Four helix bundles are also attractive for synthetic chemists because its interfaces are dominated by side chain and side chain interactions, which can be more tunable than β-strands. This study focuses on TmFtn, a naturally dimeric protein consisting of two antiparallel four helix bundles, as shown in Supplementary Fig. 1. Thermotoga maritima ferritin (TmFtn) naturally occurs as a dimer; twelve of these dimers interact with each other in a head-to-side manner to generate 24-meric hollow protein nanocage in the presence of Ca2+ or PEG. By tuning two contiguous dimeric proteins to interact in a fully or partially side-by-side fashion through protein interface redesign, we can render the self-assembly transformation of such dimeric building blocks from the protein nanocage to filament, nanorod and nanoribbon in response to multiple external stimuli.

We made a mutant named FLAL where Asn147 was replaced by aromatic phenylalanine (Phe) residue to create π–π interactions, while Glu112, Glu113, and Lys114 were replaced by three hydrophobic residues Leu, Ala, and Leu to decrease the electrostatic repulsion and increase the hydrophobic interactions between two adjacent dimers at the same time. Therefore, besides calcium ions, we also investigated the effect of PEG on the assembly behavior of FLAL molecules because PEG is a hydrophilic nonionic polymer widely used in many biochemical and pharmaceutical applications due to its mild action on the biological activity of cell components. After trying different molecular weights (PEG1000, PEG1500, and PEG3000) and concentrations (10, 20, and 30%) of PEG, we finally obtained nanorods formed in the presence of 30% PEG1500. To determine the structural basis of such nanorods, we set out to grow single crystals large enough for X-ray diffraction analyses in the presence of PEG1500. The crystal structure proved remarkably similar to the design model: protein molecules connect through designed π stacking and hydrophobic interactions in a side-by-side repeating pattern with adjacent FLAL molecules antiparallel with each other. Thus, the crystal structure is in good agreement with the above results observed by TEM, confirming the side-by-side interaction manner of dimeric FLAL molecules. Taken together, all these findings demonstrate that our protein interface redesign approach yields assembly of dimeric FLAL protein building blocks into the filaments or nanorods induced by Ca2+ or PEG rather than the inherent Ca2+-mediated 24-meric protein shell-like assembly.

>MMVISEKVRKALNDQLNREIYSSYLYLSMATYFDAEGFKGFAHWMKKQAQEELTHAMKFYEYIYERGGRVELEAIEKPPSNWNGIKDAFEAALKHEEFVTQSIYNILELASLALDHATVSFLKWFVDEQVEEEDQVREILDLLEKAFGQMSVIFQLDRYLGQRE[2x]N-methyl-3-(9H-purin-6-ylamino)benzenesulfonamide 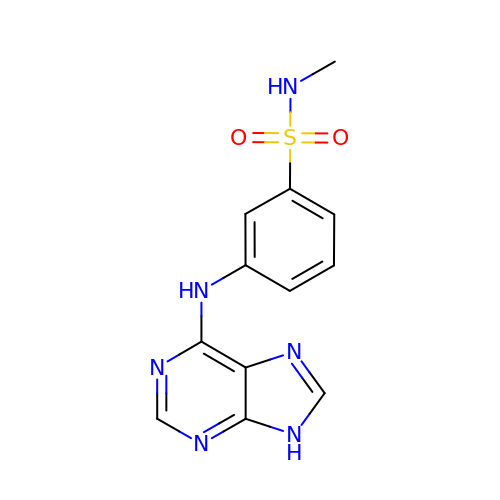| C12 H12 N6 O2 S | ONVDHHGLDDAZRU-UHFFFAOYSA-N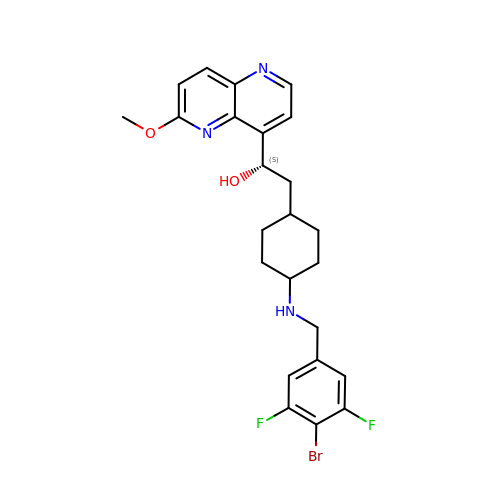(1~{S})-2-[4-[[4-bromanyl-3,5-bis(fluoranyl)phenyl]methylamino]cyclohexyl]-1-(6-methoxy-1,5-naphthyridin-4-yl)ethanol | C24 H26 Br F2 N3 O2 | RCLQISQKEHCDJQ-HTZUNMPGSA-N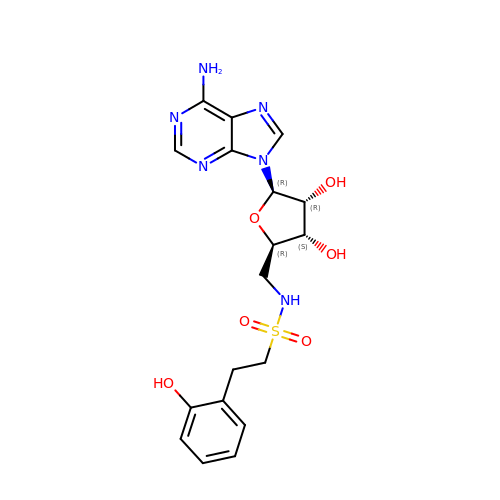5'-deoxy-5'-({[2-(2-hydroxyphenyl)ethyl]sulfonyl}amino)adenosine | C18 H22 N6 O6 S | NIEGSPNRJDKALY-SCFUHWHPSA-N> MSHPDYRMNLRPLGTPRGVSAVAGPHDIGASPGDKKSKNRSTRGKKKSIFETYMSKEDVSEGLKRGTLIQGVLRINPKKFHEAFIPSPDGDRDIFIDGVVARNRALNGDLVVVKLLPEEHWKVVKPESNDKETEAAYESDIPEELCGHHLPQQSLKSYNDSPDVIVEAQFDGSDSEDGHGITQNVLVDGVKKLSVCVSEKGREDGDAPVTKDETTCISQDTRALSEKSLQRSAKVVYILEKKHSRAATGFLKLLADKNSELFRKYALFSPSDHRVPRIYVPLKDCPQDFVARPKDYANTLFICRIVDWKEDCNFALGQLAKSLGQAGEIEPETEGILTEYGVDFSDFSSEVLECLPQGLPWTIPPEEFSKRRDLRKDCIFTIDPSTARDLDDALSCKP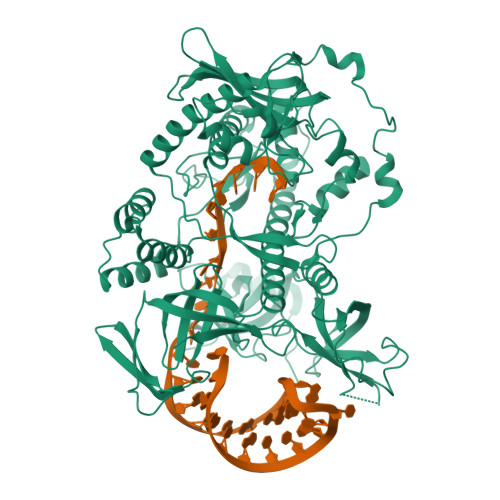LADGNFKVGVHIADVSYFVPEGSDLDKVAAERATSVYLVQKVVPMLPRLLCEELCSLNPMSDKLTFSVIWTLTPEGKILDEWFGRTIIRSCTKLSYEHAQSMIESPTEKIPAKELPPISPEHSSEEVHQAVLNLHGIAKQLRQQRFVDGALRLDQLKLAFTLDHETGLPQGCHIYEYRESNKLVEEFMLLANMAVAHKIHRAFPEQALLRRHPPPQTRMLSDLVEFCDQMGLPVDFSSAGALNKSLTQTFGDDKYSLARKEVLTNMCSRPMQMALYFCSGLLQDPAQFRHYALNVPLYTHFTSPIRRFADVLVHRLLAAALGYRERLDMAPDTLQKQADHCNDRRMASKRVQELSTSLFFAVLVKESGPLESEAMVMGILKQAFDVLVLRYGVQKRIYCNALALRSHHFQKVGKKPELTLVWEPEDMEQEPAQQVITIFSLVEVVLQAESTALKYSAILKRPGTQGHLGPEKEEEESDGEPEDSSTS> GIPIEPVLENVQPNSAASKAGLQAGDRIVKVDGQPLTQWVTFVMLVRDNPG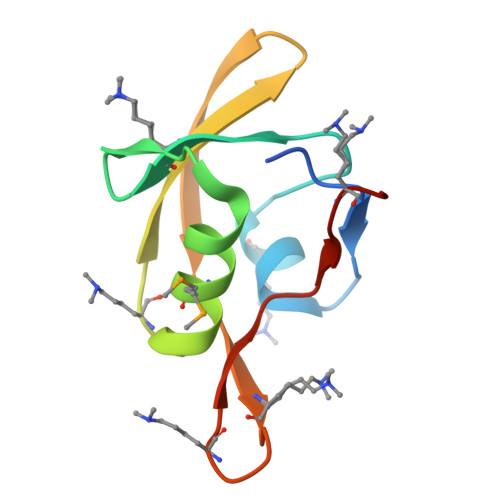KSLALEIERQGSPLSLTLIPESKPGNGKAIGFVGIEPKVI>[4x]KSKTEYYNAWSEWERNAPPGNGEQREMAVSRLRDCLDRQAHELELNNLGLSSLPELPPHLERLVASCNSLTELPELPQSLKSLEVYENNLKALPDLPPLLVDLRVFNNQLEELPELQNLPFLTEIYANNNSLKTLPDLPPSLVDLNVRENYLTALPELPQSLIFLDISDNILSGLSELPPNLSCLDASRNGIRSLCDLPPSLVYLDVRDNQLIELPALP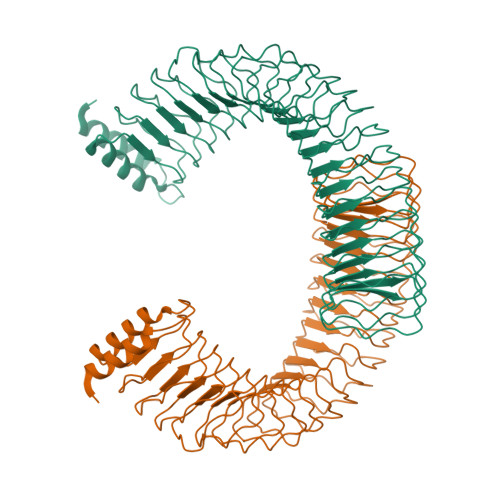SGLERLIASFNHLAELPELPPNLYYLDASRNEISSLCDLPPSLVDLNVRKNQLIELPALPPDLERLIASFNHLAELPELPPNLSYLDASRNEISSLCDLPPSLVDLNVRKNQLIELPALPPDLERLIASFNHLAELPELPPNLSYLDASRNEISSLCDLPPSLVELDVRDNQLIELPALPPHLERLIASLNHLAEVPELPQNLKQLHVEHNALREFPDIPESVEDLRMD Neuroglobin (Ngb) is a member of the globin protein family that is expressed in the brain (∼1 µM) and the retina (∼100 µM) of vertebrates. It is involved in the protection of the nervous tissue from ischemic damage via a still-elusive biochemical mechanism. Notably, Ngb is also a hexacoordinate protein in the ‘deoxy’ ferrous form, with the rate-limiting step for ligand binding being the spontaneous breakage of the distal His(E7)64–heme bond.

Moreover, the three-dimensional structure of ferric Ngb (not competent for CO/O2 binding) under increasing O2 pressure was investigated in order to find out whether internal cavities in Ngb may act as storage niches for this small gaseous reactant as observed when using Xe or Kr as probes. Therefore, diffraction data for ferric Ngb (Fe3+) were collected at 50 and 80 bar of pure molecular oxygen. This species is not competent for gaseous ligand binding, but is structurally identical within experimental error to the ferrous (Fe2+) hexacoordinate species that can bind O2 or CO. From this analysis, the hydrophobic nature of the Xe-III site surface is evident, since only two atoms out of 12 reported are polar. Therefore, the presence of O2 in the Xe-III cavity supports its role as a ligand-storage site in the context of a catalytic role for Ngb. Our data show that none of the other cavities previously identified by Xe, Kr and Ar docking, including the Xe-IV site close to the heme cavity [Fig. 5(b)], is occupied by O2 even when the pressure is raised to 80 bar. Indeed, only one (Xe-III) of the two internal Xe sites identified in Ngb hosts molecular oxygen and it coincides with the region of the Ngb cavity network that binds noble gases with the highest occupancy. We therefore hypothesize that it constitutes a preferential path for ligand migration and/or a storage site for diatomic molecules.

> RPESELIRQSWRVVSRSPLEHGTVLFARLFALEPSLLPLFQYNGRQFSSPEDSLSSPEFLDHIRKVMLVIDAAVTNVEDLSSLEEYLTSLGRKHRAVGVRLSSFSTVGESLLYMLEKSLGPDFTPATRTAWSRLYGAVVQAMSRGWDG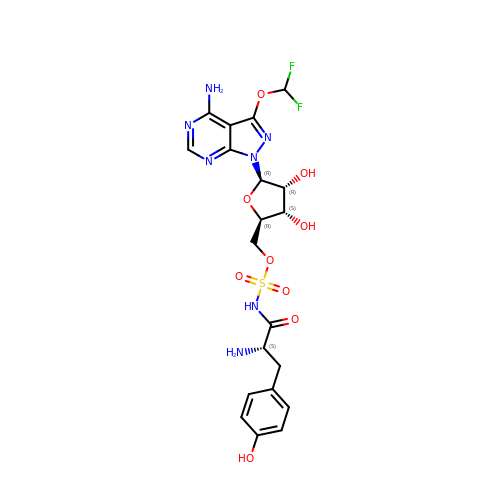{(2R,3S,4R,5R)-5-[4-amino-3-(difluoromethoxy)-1H-pyrazolo[3,4-d]pyrimidin-1-yl]-3,4-dihydroxyoxolan-2-yl}methyl [(2S)-2-amino-3-(4-hydroxyphenyl)propanoyl]sulfamate (non-preferred name) | C20 H23 F2 N7 O9 S | MUBAQGITUFCKMG-IFHUHSRSSA-N> QICPKRCVCQILSPNLATLCAKKGLLFVPPNIDRRTVELRLADNFVTNIKRKDFANMTSLVDLTLSRNTISFITPHAFADLRNLRALHLNSNRLTKITNDMFSGLSNLHHLILNNNQLTLISSTAFDDVFALEELDLSYNNLETIPWDAVEKMVSLHTLSLDHNMIDNIPKGTFSHLHKMTRLDVTSNKLQKLPPDPLFQRAQVLATSGIISPSTFALSFGGNPLHCNCELLWLRRLSREDDLETCASPPLLTGRYFWSIPEEEFLCEPPLITRHTHEMRVLEGQRATLRCKARGDPEPAIHWISPEGKLISNATRSLVYDNGTLDILITTVKDTG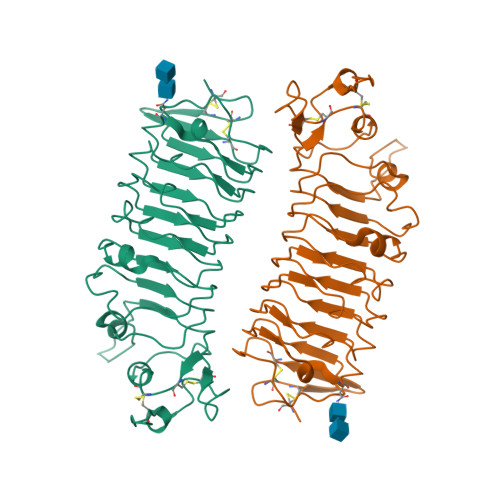AFTCIASNPAGEATQIVDLHIIKLPHHHHHH>MHHHHHHSSGRENLYFQGMSQKEQTLMTPYLQFNRHQWAALRDSVPMTLTEDEITRLKGINEDLSLEEVAEIYLPLSRLLNFYISSNLRRQAVLEQFLGTNGQRIPYIISIAGSVAVGKSTTARVLQALLSRWPEHRHVELITTDGFLHPNSVLKERGLMKKKGFPQSYDMHRLVKFVSDLKSGVPQATAPVYSHLIYDVIPDGDKTVAQPDILILEGLNVLQSGMDYPHDPHHVFVSDFVDFSIYVDAPEELLKSWYINRFLKFREGAFTDPDSYFHNYAKLSKEEAVDIATSLWNEINLMNLK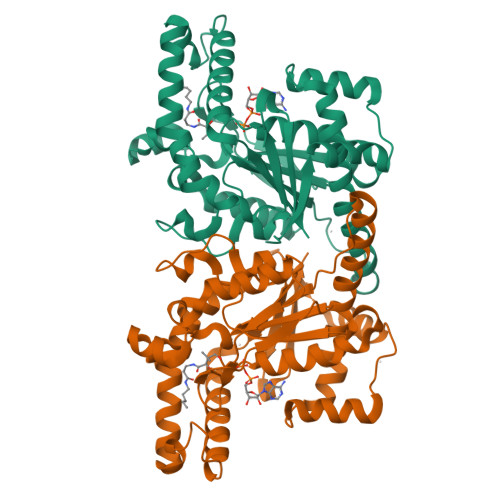ENILPTRERASLIMTKSANHSVNQVRLRK[8x]Alanine racemase (Alr) is a pyridoxal 5′-phosphate-dependent enzyme that catalyzes the racemization of l-alanine to d-alanine. Alr is one of the two targets of the broad-spectrum antibiotic d-cycloserine (DCS), a structural analogue of d-alanine. We demonstrated that Alr plays a central role in DCS resistance in M. tuberculosis, and identified that mutation of Asp 322 to Asn (D322N) confers resistance to DCS. Kinetic characterization of the D322N variant showed that this alteration reduces the affinity (Ki) of Alr for DCS 240-fold.

Comparing wild-type MtAlr to the D322′N variant, we observe a clear conformational change in the orientation of the N322′ side-chain with respect to the wild-type D322′. In particular, the χ1 angle changes from a positive value of +60.3° for D322′ to a negative value of −69.7° for N322′, as measured in chain B. Interestingly, a χ1 value of ∼ +61.0° is statistically observed in only 10% of the aspartate side-chains in crystal structures compared to a 51% probability of a −71.0° χ1 value. This less energetically favored conformation is likely to be induced by the electrostatic repulsion that a D322′ with a χ1 ∼ −71.0° would experience with the nearby fully conserved aspartate D294′, due to the short distance of about 3 Å between them and the absence of neutralizing interactions. The abolition of such repulsion in MtAlr D322N allows N322′ to acquire a more energetically favorable negative χ1 value. Therefore, rather than being oriented toward PLP and W90, like the wild-type D322′, the N322′ side chain is oriented toward D294′, with N322′ making a H-bond to D294′, at 2.99 Å. As a consequence, although the water molecule (w1) originally bridging D322′ and PLP phenolic oxygen is structurally conserved in the variant and still makes a hydrogen bond to PLP, due to the longer distance the H-bond to N322′ is no longer present. The interaction between PLP oxygen and Q323′, mediated by two water molecules, is maintained in MtAlr D322N (not shown). The crystal structures determined at high-resolution identify a change in the orientation of N322′, as compared to D322′, and the loss of a strong H-bond, as the likely cause of the observed lower affinity of MtAlr D322N for DCS.

>[2x]GSHMTPISQTPGLLAEAMVDLGAIEHNVRVLREHAGHAQLMAVVKADGYGHGATRVAQTALGAGAAELGVATVDEALALRADGITAPVLAWLHPPGIDFGPALLADVQVAVSSLRQLDELLHAVRRTGRTATVTVKVDTGLNRNGVGPAQFPAMLTALRQAMAEDAVRLRGLMSHMVYADKPDDSINDVQAQRFTAFLAQAREQGVRFEVAHLSNSSATMARPDLTFDLVRPGIAVYGLSPVPALGDMGLVPAMTVKCAVALVKSIRAGEGVSYGHTWIAPRDTNLALLPIGYADGVFRSLGGRLEVLINGRRCPGVGRICMNQFMVDLGPGPLDVAEGDEAILFGPGIRGEPTAQDWADLVGTIHYEVVTSPRGRITRTYREAENR>[5x]MDYLF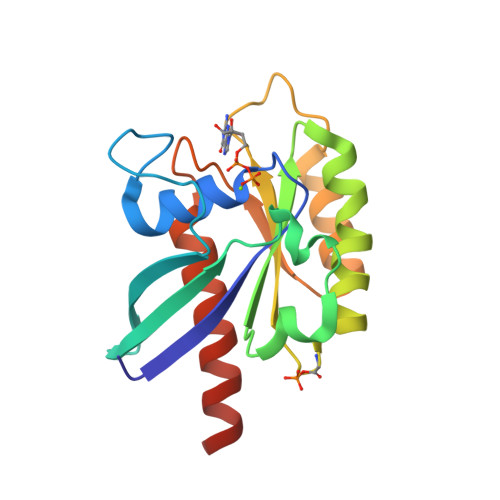KLLLIGDSGVGKTCVLFRFSEDAFNSTFISTIGIDFKIRTIELDGKRIKLQIWDTAGQERFRTITTAYYRGAMGIMLVYDITNEKSFDNIRNWIRNIEEHASADVEKMILGNKCDVNDKRQVSKERGEKLALDYGIKFMETSAKANINVENAFFTLARDIKAKMDKKHHHHHH> GAGCAGACGTG;> ACA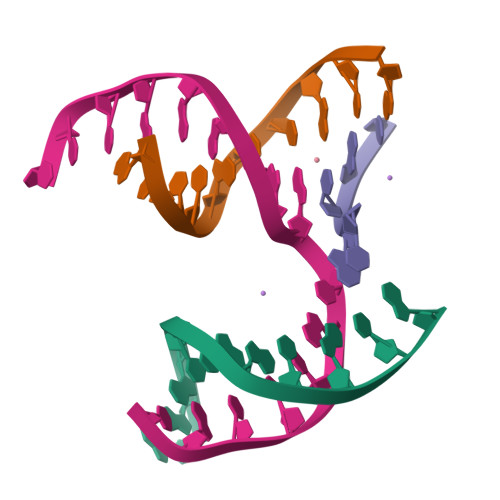CCACTCA;> CATGT;> TCTGAGTGGCGTCTGC> KPKLLNKFDKTIKAELDAAEKLRKRGKIEEAVNAFKELVRKYPQSPRARYGKAQCEDDLAEKRRSNEVLRGAIETYQEVASLPDVPADLLKLSLKRRSDRQQFLGHMRGSLLTLQRLVQLFPNDTSLKNDLGVGYLLIGDNDNAKKVYEEVLSVTPNDGFAKVHYGFILKAQNKIAESIPYLKEGIESGDPGTDDGRFYFHLGDAMQRVGNKEAYKWYELGHKRGHFASVWQRSLYNVNGLKAQPWWTPKETGYTELVKSLERNWKLIRDEGLAVMDKAKGLFLPEDENLREKGDWSQFTLWQQGRRNENACKGAPKTCTLLEKFPETTGCRRGQIKYSIMHPGTHVWPHTGPTNCRLRMHLGLVIPKEGCKIRCANETKTW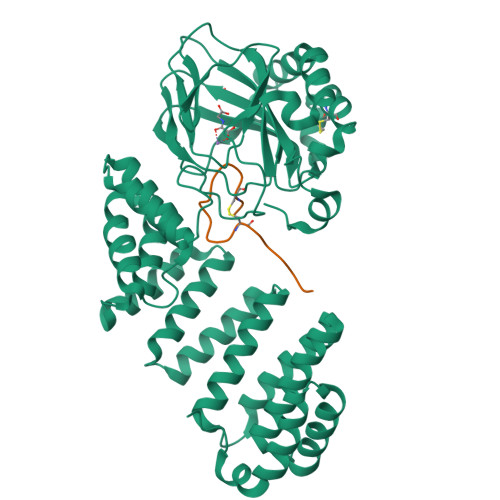EEGKVLIFDDSFEHEVWQDASSFRLIFIVDVWHPELTPQQRRSLPAI;> DGDQCETSPCQNQGKCKDGLGEYTCTCLEGFEGKNCELF> SRSF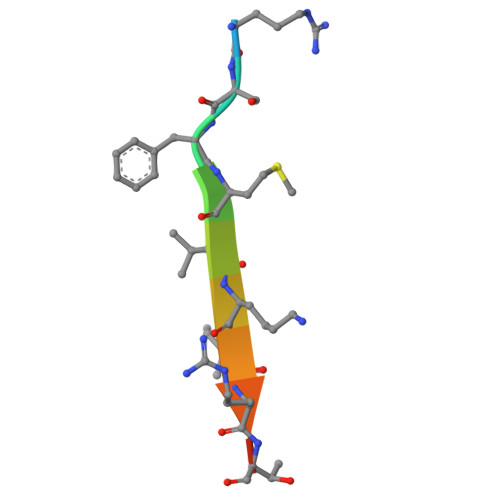MVKIRTKN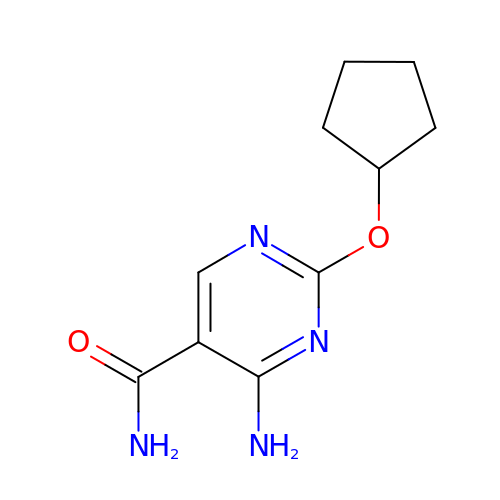4-amino-2-(cyclopentyloxy)pyrimidine-5-carboxamide | C10 H14 N4 O2 | YTVJKSRJMDSHEP-UHFFFAOYSA-N> HHHHHHHSEMTPREIVSELDKHIIGQDNAKRSVAIALRNRWRRMQ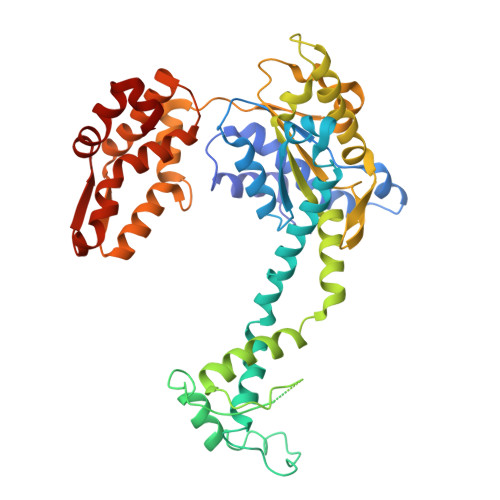LNEELRHEVTPKNILMIGPTGVGKTEIARRLAKLANAPFIKVEATKFTEVGYVGKEVDSIIRDLTDAAVKMVRVQAIEKNRYRAEELAEERILDVLIPPAKNNWGQTEQQQEPSAARQAFRKKLREGQLDDKEIEIDLAAAPMGVEIMAPPGMEEMTSQLQSMFQNLGGQKQKARKLKIKDAMKLLIEEEAAKLVNPEELKQDAIDAVEQHGIVFIDEIDKICKRGESSGPDVSREGVQRDLLPLVEGCTVSTKHGMVKTDHILFIASGAFQIAKPSDLIPELQGRLPIRVELQALTTSDFERILTEPNASITVQYKALMATEGVNIEFTDSGIKRIAEAAWQVNESTENIGARRLHTVLERLMEEISYDASDLSGQNITIDADYVSKHLDALVADEDLSRFIL>[4x]MTKTKFEKVLLIVNPKAGQGDLH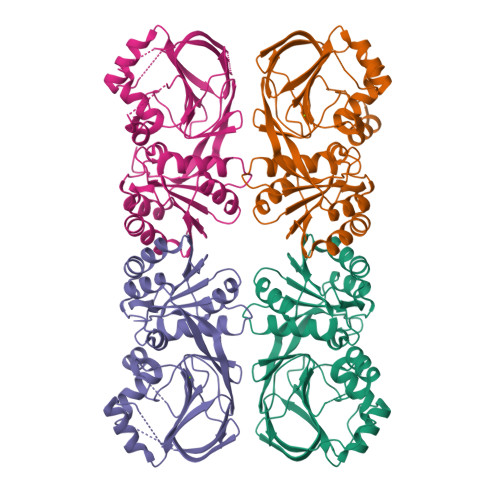TNLTKIVPPLAAAFPDLHILHTKEQGDATKYCQEFASKVDLIIVFGGDGTVFECTNGLAPLEIRPTLAIIPGGTCNDFSRTLGVPQNIAEAAKLITKEHVKPVDVAKANGQHFLNFWGIGLVSEVSNNIDAEEKAKLGKIGYYLSTIRTVKNAETFPVKITYDGQVYEDEAVLVMVGNGEYLGGIPSFIPNVKCDDGTLDIFVVKSTGIQAFKDYIGKKLFEDSNENDIFHVKAKSIHIETEEEKEVDTDGESSLHTPCQIELLQGHFTMIYNPAVV>GGWIRNIGRYLSYLVDDTFEEYAYDVVDGIAKARTQEELLEGVYKALRLAPKLKKKAESKGCPPPRIPSPEDIEALEEKVEQLSNPKDLRKLAVSLALWAFASWNNCP[7x];>[10x]MYVRISGRIRLNAHSLNAQGGGGTNYIEITKTKVTVRTENGWTVVEVPAITGNMLKHWHFVGFVDYFKTTPYGVNLTERALRYNGTRFGQGETTATKANGATVQLNDEATIIKELADADVHGFLAPKTGRRRVSLVKASFILPTEDFIKEVEGERLITAIKHNRVDVDEKGAIGSSKEGTAQMLFSREYATGLYGFSIVLDLGLVGIPQGLPVKFEENQPRPNIVIDPNERKARIESALKALIPMLSGYIGANLARSFPVFKVEELVAIASEGPIPALVHGFYEDYIEANRSIIKNARALGFNIEVFTYNVDLGEDIEATKVSSVEELVANLVKMV;> MDILLVCLRFPFFSVAKRSYQVRTSFLLPPPSALKGALAKGLILLKPEKYASSSLDEAALKAIKEIESKLVDIKAVSVAPLSPLIRNAFLLKRLRNLESGSNAEKSDAMRREYTFTRELLVAYIFKNLTQEEKNLYLKAAMLIDVIGDTESLATPVWASFVKPEDKKAPLAFSAPYTEIYSLLSSKIQAKGKIRMYIEKMRVSPEYSKTKGPQEEIFYLPIEERRYKRIVYYARIYPPEVEKALTV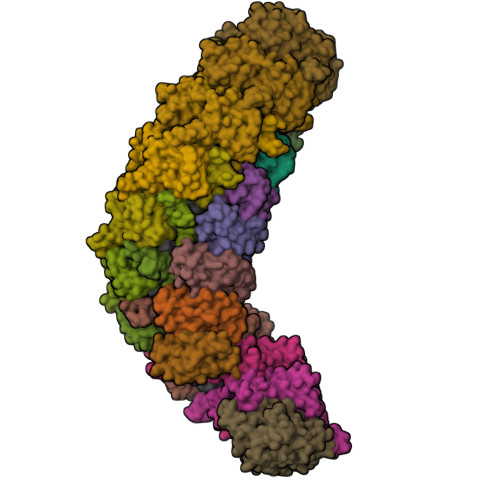DGEVLGIWIP> GASTVEKELLRSRRLENSIIEQKGTMRCYAYVMEQNLPENLLFDYENGVITQGLSEHVYKFNRVIPHLKVSEDKFFTQEYSVYHDMCLNQKKNFNLISLSTTPHGSLRESLIKFLAEKDTIYQKQYVITLQFVFLSDDEFSQDMLLDYSHNDKDSIKLKFEKHSISLDSKLVIIENGLEDLPLNFSCDEHPNLPHSGMG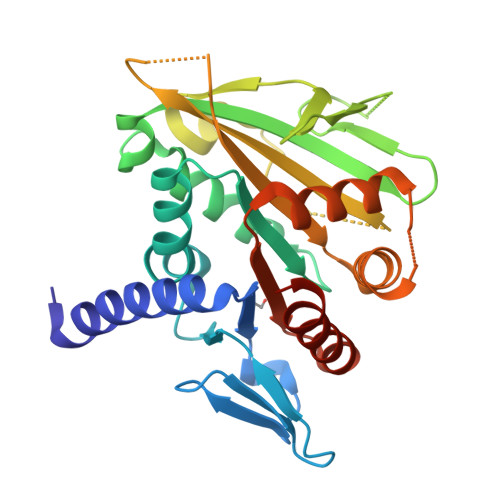IIKVQFFPRDSKSDGNNDPVPVDFYFIELNNLKSIEQFDKSIFKKESCETPIALVLKKLISDTKSFFLLNLNDSKNVNKLLTISEEVQTQLCKRKKKLT> MYRYEKKGPKRGVALYSYSAEFGLTKTLEDCFEDLHDMGAHGIEILANTHIENYPYPTDEWVEKWWRLCDKYEIVPVEYGNWIDSHVLGDRDLTTEESVEMLKRDIRLAHRLGFTVMRTKMPVINDLLEPVENWKEIIKGALPLAEELGIKMCPEIHTPSNLKGKLVNDFVEFIKETGTKNFGLNIDFSVFRTSFAEGEWVDPNYTPNKPEDIIPLLPYVYCCHAKFIHMSDDFKETTIPYEEVVKTMEDNGYEGYLLSEYEGADKYDEGYEVGQTLRKHHILLKNLLGD;> MEKQVIQSVGFRNIKNGNGEITGFQFKVKLPYYRGVFLSQIRPGTLFVDGQKIEKDQITWTINGEEYTNQEMRGDFKTHWATTKPAVLKVKMPGGLAQGYHDLKYGFCFTSSYMPPIIQDGLDPDKESMVYMPEFGHHVNERRLLIVKLAAALEHHHHHH

Here, we present the identification and structural basis for the activation of xenobiotic C-glycosides by heterocomplex C-deglycosylation enzymes from intestinal and soil bacteria. They are found to be metal-dependent enzymes exhibiting broad substrate specificity toward C-glycosides. DgpA catalyzes the oxidation of the glucoside moiety of puerarin to generate 3”-oxo-puerarin, in which the 3”-oxo-sugar moiety is cleaved by an unusual C-deglycosylation enzyme complex, which is an α4β4 heterooctamer of DgpB-C, to produce daidzein. For clarity, the DgpB-C and DfgA-B complexes are referred to as PuCGD and EuCGD, respectively.

To elucidate the molecular basis of the enzymatic C-C bond cleavage reaction in the activation/inactivation of xenobiotic compounds by CGDs, we solved the apo structures of PuCGD, EuCGD, and AgCGD2, and the co-substrate structure of AgCGD2 with homoorientin, at 2.50, 2.40, 2.30 and 2.25 Å resolution, respectively. While these three CGDs shared similar heterodimer unit structures, PuCGD and EuCGD formed α4β4 heterooctamers and AgCGD2 formed an αβ heterodimer. The heterodimer structures of EuCGD and AgCGD2 were similar to that of PuCGD, with RMSD values of 2.2 and 3.5 Å, respectively. The major structural differences among these enzymes lay on the interface between the α- and β-subunits; the α-subunits of PuCGD and AgCGD2 (represented as PuCGDα and AgCGD2α, respectively) were composed of a TIM barrel domain and an additional domain with four α-helices (lid domain), which was not observed in EuCGDα. Instead, the loop between M121-N133 of EuCGDα, forming the active site cavity, was six residues longer than those of PuCGDα and AgCGD2α. Moreover, the N-terminal loops of EuCGDβ and AgCGD2β were also short as compared to that of PuCGDβ. On the other hand, 11 residues were inserted in the loop between β7 and β8 of EuCGDβ (T110-V139), as compared to those of PuCGDβ and AgCGD2β, and the loop was involved in the formation of the active site cavity. The difference anomalous Fourier maps of AgCGD2, PuCGD, and EuCGD suggested that these enzymes contain Mn2+ as a metal ion in the active site. In contrast, EuCGD acted on C6-glycosylated compounds 3-5, but not on C8-glycosylated compounds 1 and 2. In the model of EuCGD with orientin, furthermore, the B-ring of orientin also clashed with active site residues including Leu128α and Pro115β.> EPCVEVVPNITYQCMELNFYKIPDNLPFSTKNLDLSFNPLRHLGSYSFFSFPELQVLDLSRCEIQTIEDGAYQSLSHLSTLILTGNPIQSLALGAFSGLSSLQKLVAVETNLASLENFPIGHLKTLKELNVAHNLIQSFKLPEYFSNLTNLEHLDLSSNKIQSIYCTDLRVLHQMPLLNLSLDLSLNPMNFIQPGAFK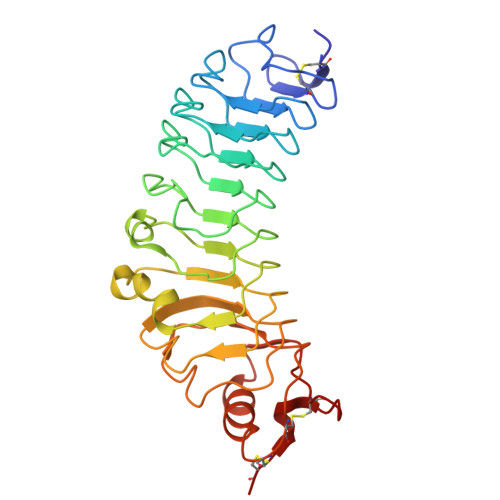EIRLKELALDTNQLKSVPDGIFDRLTSLQKIWLHTNPWDCSCPRIDYLSRWLNKNSQKEQGSAKCSGSGKPVRSIICP>CGAMSTAIKKRNLEVKTQMSETIWLEPASERTVFLQIKNTSDKDMSGLQGKIADAVKAKGYQVVTSPDKAYYWIQANVLKADKMDLRESQGWLNRGYEGAAVGAALGAGITGYNSNSAGATLGVGLAAGLVGMAADAMVEDVNYTMITDVQIAE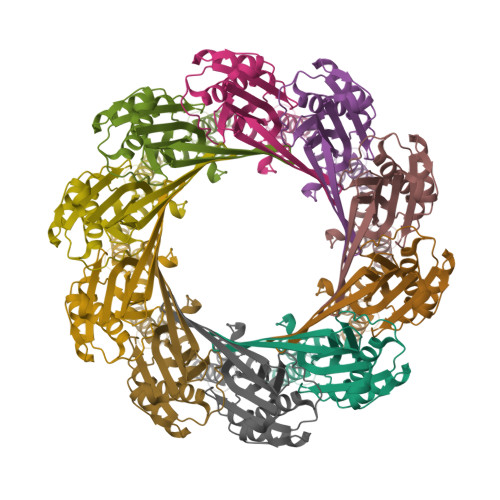RTKATVTTDNVAALRQGTSGAKIQTSTETGNQHKYQTRVVSNANKVNLKFEEAKPVLEDQLAKSIANILGS[10x]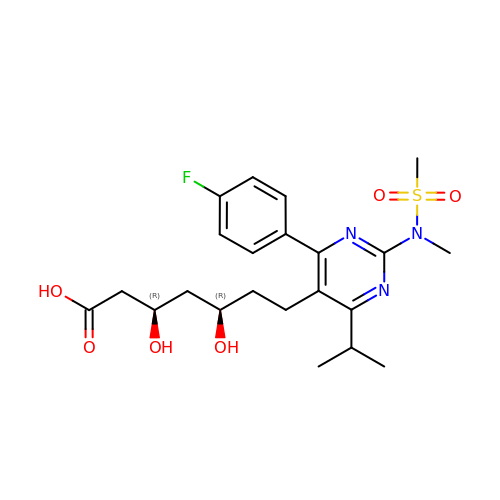7-[4-(4-FLUORO-PHENYL)-6-ISOPROPYL-2-(METHANESULFONYL-METHYL-AMINO)-PYRIMIDIN-5-YL] -3,5-DIHYDROXY-HEPTANOIC ACID | C22 H30 F N3 O6 S | ZVPAUNJUMAQCNK-IAGOWNOFSA-N>MSFNTIIDWNSCTAEQQRQLLMRPAISASESITRTVNDILDNVKARGDEALREYSAK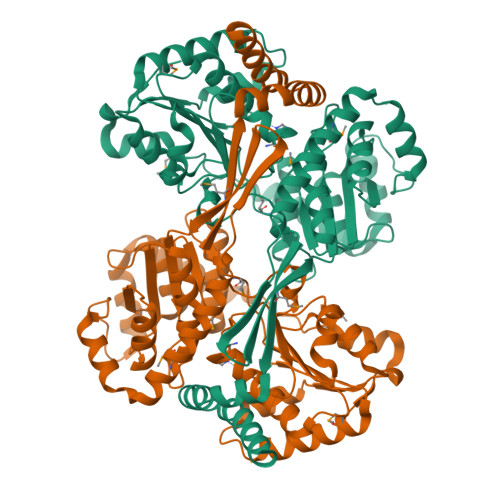FDKTTVTALKVSAEEIAAASERLSDELKQAMAVAVKNIETFHTAQKLPPVDVETQPGVRCQQVTRPVASVGLYIPGGSAPLFSTVLMLATPASIAGCKKVVLCSPPPIADEILYAAQLCGVQDVFNVGGAQAIAALAFGTESVPKVDKIFGPGNAFVTEAKRQVSQRLDGAAIDMPAGPSEVLVIADSGATPDFVASDLLSQAEHGPDSQVILLTPAADMARRVAEAVERQLAELPRAETARQALNASRLIVTKDLAQCVEISNQYGPEHLIIQTRNARELVDSITSAGSVFLGDWSPESAGDYASGTNHVLPTYGYTATCSSLGLADFQKRMTVQELSKEGFSALASTIETLAAAERLTAHKNAVTLRVNALKEQA[2x]> MARGLNQVFLIGTLTARPDMRYTPGGLAILDLNLAGQDAFTDESGQER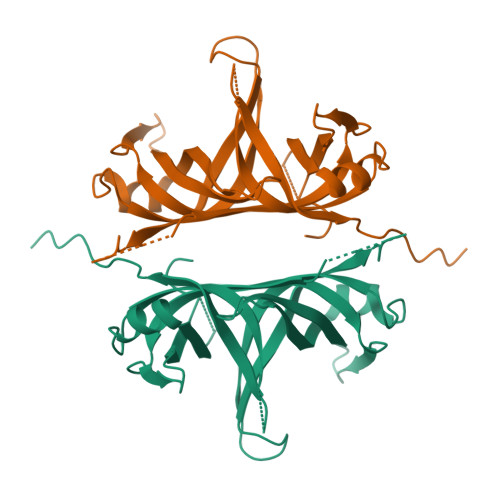EVPWYHRVRLLGRQAEMWGDLLEKGQLIFVEGRLEYRQWEKDGEKKSEVQVRAEFIDPLEGRGRETLEDARGQPRLRRALNQVILMGNLTRDPDLRYTPQGTAVVRLGLAVNERRRGQEEERTHFLEVQAWRELAEWASELAKGDGLLVIGRLVNDSWTSSSGERRFQTRVEALRLERPLEDFPPEEDLPF> VNPKRSANINKLRESGNAEYRK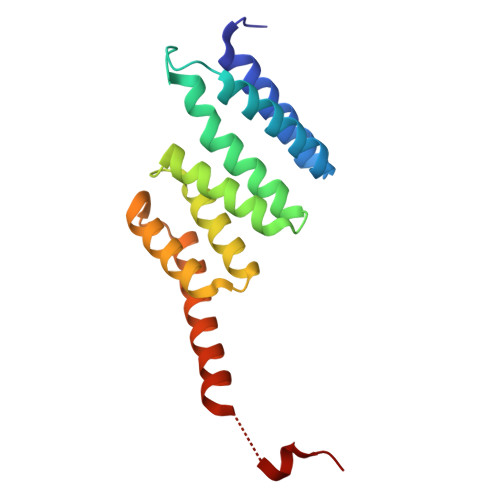QRYGDAIKLYTLGLQMALTRPAWEPAGLVRDEIHQLYSNRAQAYMQLGQWPEAAADAECSVEAKRQGNAKAWYRRGKCLMEMRRLQEAREWVARGLEFEGEEKELAELLKEIDSKLAAEKASRDAHDNDGPTVEEVD>[4x]MAAKKDYYAILGVPRNATQEEIKRAYKRLARQYHPDVNKSPEAEEKFKEINEAYAVMSDPEKRRIYDTYGTTEAPPPPPPGGYDFSGFDVEDFSEFFQELFGPGLFGKGRDLRAELPLTLEEAFHGGERVVEVAGRRVSVRMPPGVREGSVIRVPGMGGQGNPPGDLLLVVRMLPHPVFRLEGQDLYATLDVPAPIAVVGGKVRAMTLEGPVEVAVPPRTQAGRKMRLKGGGFPGPAGRGDLYLEVRITIPERLTPEEEALWKKLAEAYYARAAAALEHHHHHH

DnaJ protects the cell from adverse conditions through the prevention of protein aggregation or by assisting the refolding of unfolded proteins and is an essential partner of the chaperone DnaK in bacterial DnaK–DnaJ–GrpE chaperone systems. DnaJ, the bacterial homologue of Hsp40, stimulates ATP hydrolysis by DnaK (Hsp70) and thus mediates capture of substrate protein, but is also known to possess chaperone activity of its own. T. thermophilus DnaJ is a typical type II DnaJ, i.e. it lacks the zinc-finger domains found in type I DnaJs such as that of E. coli. Crystal structures of the complete molecular cochaperone DnaJ from Thermus thermophilus comprising the J, GF and C-terminal domains and of the J and GF domains alone showed an ordered GF domain interacting with the J domain.

The electron-density map of this structure inspired a third construct, this time of a complete DnaJ from which a disordered stretch of seven amino acids (108–114 in the linker between the GF domain and C-terminal domain; DnaJΔ108–114) was deleted with a view to increasing conformational stability. Therefore, a full-length construct was prepared that lacked the 108–114 stretch (DnaJΔ108–114), which was shown to be functional in refolding assays. The subsequent substitution of four residues with methionine (construct DnaJΔ108–114/4M) allowed SeMet-SAD phasing, resulting in the determination of the first crystal structure of a complete functional DnaJ containing J, GF and C-terminal domains to 2.9 Å resolution. In all four monomers in the asymmetric unit of the DnaJΔ108–114 crystals the orientation of the C-terminal and J/GF domains differs, showing that the Δ108–114 deletion does not restrict their mutual motion. Moreover, the J/GF regions of chains B and D showed poor electron density, also indicating flexibility. Since the J/GF domains visible in the DnaJΔ108–114 crystal structure each assume a different orientation relative to their respective C-terminal domains, it seems likely that this flexibility is, at least to a large extent, concentrated at the junction between the J/GF domain and the C-terminal domain.>GAMGSGIQMKEEASEHGGSADETQELSPVSDSSDEMPNNAKRRRRSQSMIANKRIHQAFQEDEGDEDWEEEEHKPKAKRRYNTRSNESFSEGDDEPFEVSESSALEDELSDSEDSFIRSVRSKPKYKPGTRRSTRLRNRRSQDEEESEEEHRPILRERTSRINYSVPLAFPPVDEMDGDPSSQVNQSRSRKTHSELAITKLLRQQVSSFMPYIDSSGSESESDNTRIKKSSAKTIKALTDPANSGGPPDFGRIREKSDLADSDPLGVDSSLSFESVGGLDNYINQLKEMVMLPLLYPEIFQRFNMQPPRGVLFHGPPGTGKTLMARALAAACSSENKKVSFYMRKGADCLSKWVGEAERQLRLLFEEAKSTQPSIIFFDQIDGLAPVRSSKQEQIHASIVSTLLALMDGMESRGQVIIIGATNRPDAVDPALRRPGRFDREFYFPLPDRDARKKIIEIHTRNWDPPVPEWLCSMLAEKSKGYGGADLRALCTEAALNSIKRTYPQLYRSTKRLQIDPKTIKVKVKDFVMSMKRMIPSSERSSISPSKPLSPELKPLLNEAFQDIEKTLQKLMPVASKLNPLEEVMYDDPKENDFEYQQRLETFETLRIYKPRFLICGRKGLGQTALGPAILQQYEGVHVQSFDMSTLLQDSTQSIETSIIHLFLEVRRHTPSIIYIPDIDNWLNVLPLTAITTFSSMLERLDFSDQILFLALSSSPLSELHPQLREWFSSKQSVYSLQYPTRDSIIAFFQPILELIKASPTELPGGIPRKRRVLPELPLAPDPPPFTSQKITLKQTKQADMRLLNKLKIKLNALLGSLRARYRKFKKPLIDFNDIYCVDPETGHSYRSREECHYEFVDDVVKQIGSDQKFSMMSLEEIEKRTWDNCYCTPKQFVHDIKLILRDALQLEDSETIKRAQEMYANVLLGVEDMEDDQFSQRCERMALREAERRKLRHGKLQKHLDETKADMQFTSEKPSVDESITEVDDAIKDGPPVLAETLTNSLMEDVGPENVDMDIEDNEIFTNQSTMSVPSMLVENEESPKPDEYIDQKDKVQSPLLNGKSPVGVPSEAALRVSTDVSTNISSNGRADIPVDTLITSPADVPNNAPTDAHNITSADGHIENIEQEVVFPDLVFDEDRLTPLKQLLIDSTTGFTVDQLLHLHSFLYQIIWNTKSEWNRNSVVDECERAVKEFMINALQ[6x]

ATAD2 (also termed ANCCA) is a histone chaperone that has been implicated in nucleosome density regulation by histone H3–H4 loading or removal. Although histone chaperones responsible for nucleosome assembly and disassembly usually do not contain ATPase domains, ATAD2 is unique because it is the only known AAA+ ATPase histone chaperone. Here, we demonstrate ATP-dependent histone H3–H4 deposition onto DNA by Abo1, the fission yeast ortholog of ATAD2, using an in vitro single-molecule imaging technique, the DNA curtain. We solve the cryo-EM structures of Abo1 in three different nucleotide states (apo, ADP, and ATP), revealing a major reorganization of the AAA+ domains from an open spiral to a closed ring—a structural change that can also be recapitulated in real time by high-speed atomic force microscopy (HS-AFM).

We first solved the cryo-EM structure of Abo1 in an ATP-bound state to 3.5 Å resolution using an ATP-hydrolysis deficient Abo1 Walker B mutant (E372Q). The atomic resolution model revealed two layers of AAA+ domains arranged in a hexameric spiral, with the AAA1 domains forming the top layer and the AAA2 domains the bottom layer. Densities for six bound nucleotides were found at the interface of AAA1 protomers. We assigned five of the nucleotide densities as ATP, but the identity of one nucleotide (in subunit A) could not be determined with certainty although we modeled this nucleotide as ADP based on superposition with the ADP state (see below). No nucleotide density was found at the interface of the AAA2 domains, consistent with the fact that AAA2 has no consensus Walker A or B motifs and is presumably catalytically inactive. First, Abo1 subunits have a molecular clasp where the “knob” of one subunit locks into a “hole” of the neighboring subunit by an electrostatic interaction. However, individual subunits in the ATP state displayed a marked difference where the AAA1 domain and the linker arm progressively shift away from the AAA2 domain as the subunits rise in height along the spiral axis. Unexpectedly, after building an atomic model into the cryo-EM map of the ATP-Abo1, we discovered a lobe of extra density in the central pore that could not be accounted for by any part of Abo1. We modeled this density as a 14-alanine chain, and examination of interactions between the polyalanine chain and Abo1 revealed that the W345 sidechains of Abo1 form a winding tryptophan staircase around the peptide, where the middle subunits (B–E) form direct contacts. In the ATP-state, Abo1 assumes a closely packed spiral that binds the histone H3 N-terminal through its pore loops and the histone body through its bromodomain.> VIHLDSKNFDSFLASHEIAVVDFWAEWCAPCLILAPIIEELAEDYPQ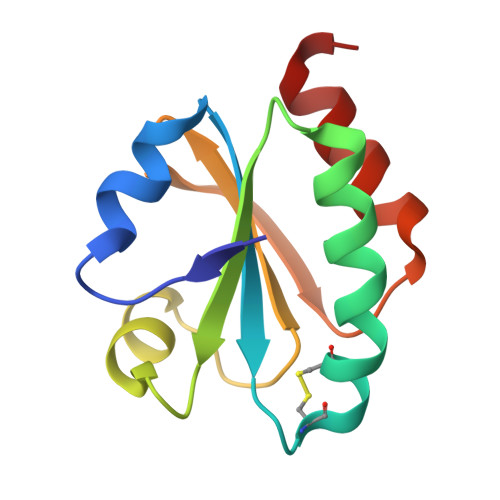VGFGKLNSDENPDIAARYGVMSLPTVIFFKDGEPVDEIIGAVPREEIEIRIKNLLGE>MADLEAVLADVSYLMAMEKSKATPAARASKKILLPEPSIRSVMQKYLEDRGEVTFEKIFSQKLGYLLFRDFCLKHLEEAKPLVEFYEEIKKYEKLETEEERLVCSREIFDTYIMKELLACSHPFSKSAIEHVQGHLVKKQVPPDLFQPYIEEICQNLRGDVFQKFIESDKFTRFCQWKNVELNIHLTMNDFSVHRIIGRGGFGEVYGCRKADTGKMYAMKCLDKKRIKMKQGETLALNERIMLSLVSTGDCPFIVCMSYAFHTPDKLSFILDLMNGGDLHYHLSQHGVFSEADMRFYAAEIILGLEHMHNRFVVYRDLKPANILLDEHGHVRISDLGLACDFSKKKPHASVGTHGYMAPEVLQKGVAYDSSADWFSLGCMLFKLLRGHSPFRQHKTKDKHEIDRMTLTMAVELPDSFSPELRSLLEGLLQRDVNRRLGCLGRGAQEVKESPFFRSLDWQMVFLQKYPPPLIPPRGEVNAADAFDIGSFDEEDTKGIKLLDSDQELYRNFPLTISERWQQEVAETVFD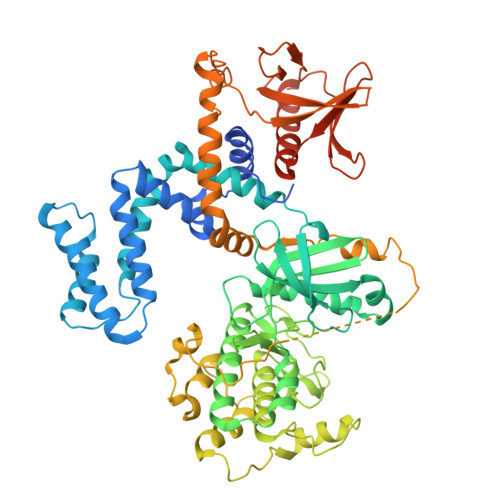TINAETDRLEARKKTKNKQLGHEEDYALGKDCIMHGYMSKMGNPFLTQWQRRYFYLFPNRLEWRGEGEAPQSLLTMEEIQSVEETQIKERKCLLLKIRGGKQFVLQCDSDPELVQWKKELRDAYREAQQLVQRVPKMKNKPRAPVVELSKVPLIQRGSANGL[4x]> MEALIPVINKLQDVFNTVGADIIQLPQIVVVGTQSSGKSS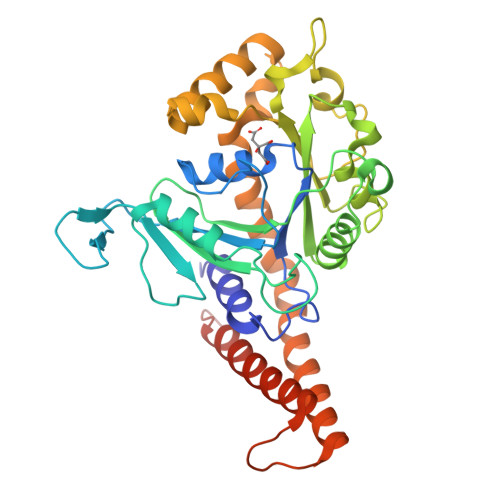VLESLVGRDLLPRGTGIVTRRPLILQLVHVSQEDKRKTTGEENGVEAEEWGKFLHTKNKLYTDFDEIRQEIENETERISGNNKGVSPEPIHLKIFSPNVVNLTLVDLPGMTKVPVGDQPKDIELQIRELILRFISNPNSIILAVTAANTDMATSEALKISREVDPDGRRTLAVITKLDLMDAGTDAMDVLMGRVIPVKLGIIGVVNRSQLDINNKKSVTDSIRDEYAFLQKKYPSLANRNGTKYLARTLNRLLMHHIRDCLPELKTRINVLAAQYQSLLNSYGEPVDGSGSGSGSKEAADMLKALQGASQIIAEIRETHLWLEHHHHHH> MFAGLQDLGVANGEDLKETLTNCTEPLKAIEQFQTENGVLLPSLQSALPFLDLHGTPRLEFHQSVFDELRDKLLERVSAIASEGKAEERYKKLEDLLEKSF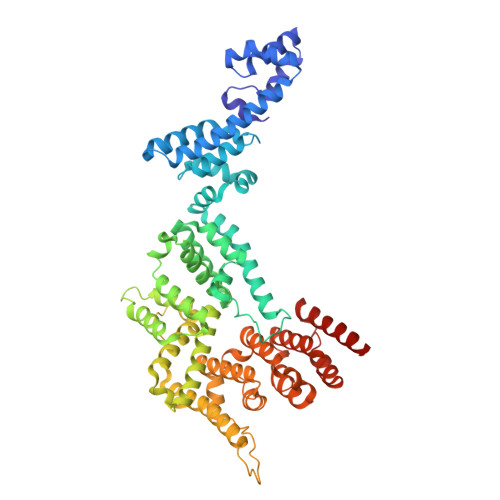SLVKMPSLQPVVMCVMKHLPKVPEKKLKLVMADKELYRACAVEVKRQIWQDNQALFGDEVSPLLKQYILEKESALFSTELSVLHNFFSPSPKTRRQGEVVQRLTRMVGKNVKLYDMVLQFLRTLFLRTRNVHYCTLRAELLMSLHDLDVGEICTVDPCHKFTWCLDACIRERFVDSKRARELQGFLDGVKKGQEQVLGDLSMILCDPFAINTLALSTVRHLQELVGQETLPRDSPDLLLLLRLLALGQGAWDMIDSQVFKEPKMEVELITRFLPMLMSFLVDDYTFNVDQKLPAEEKAPVSYPNTLPESFTKFLQEQRMACEVGLYYVLHITKQRNKNALLRLLPGLVETFGDLAFGDIFLHLLTGNLALLADEFALEDFCSSLFDGFFLTASPRKENVHRHALRLLIHLHPRVAPSKLEALQKALEPTGQSGEAVKELYSQLGEKLEQLDHRKPSPAQ> MQTLKELIASNPDDLTTELKRAFRPL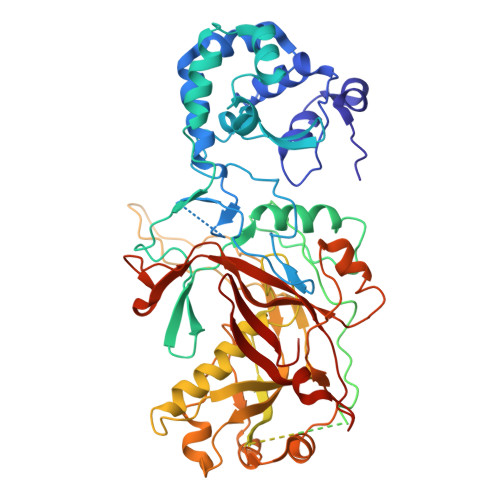TPHIAIDGNELDALTILVNLTDKTDDQKDLLDRAKCKQKLRDEKWWASCINCVNYRQSHNPKFPDIRSEGVIRTQALGELPSFLLSSSKIPPYHWSYSHDSKYVNKSAFLTNEFCWDGEISCLGELLKDADHPLWNTLKKLGCSQKTCKAMAKQLADITLTTINVTLAPNYLTQISLPDSDTSYISLSPVASLSMQSHFHQRLQDENRHSAITRFSRTTNMGVTAMTCGGAFRMLKSGAKFSSPPHHRLNSKRSWLTSEHVQSLKQYQRLNKSLIPENSRIALRRKYKIELQNMVRSWFAMQDHTLDSNILIQHLNHDLSYLGATKRFAYDPAMTKLFTELLKRELSNSINNGEQHTNGSFLVLPNIRVCGATALSSPVTVGIPSLTAFFGFVHAFERNINRTTSSFRVESFAICVHQLHVEKRGLTAEFVEKGDGTISAPATRDDWQCDVVFSLILNTNFAQHIDQDTLVTSLPKRLARGSAKIAIDDFKHINSFSTLETAIESLPIEAGRWLSLYAQSNNNLSDLLAAMTEDHQLMASCVGYHLLEEPKDKPNSLRGYKHAIAECIIGLINSITFSSETDPNTIFWSLKNYQNYLVVQPRSINDETTDKSSL> AMENKIEVNNKDEMNRWFEEFKKGNGLVDTFTNSYSFCESIPNLDRFVFQMASATDDAQKDSIYASALVEATKFCAPIYECAWVSSTGIVKKGLEWFEKNAGTIKSWDESYTELKVDVPKIEQLTGYQQAALKWRKDIGFRVNANTAALSNKVLAEYKVPGEIVMSVKEMLSDMIRRRNLILNRGGDENPRGPVSHEHVDWCREFVKGKYIMAFNPPWGDINKSGRSGIALVATGLAKLAETEGKGIFDEAKKTVEALNGYLDKHKDEVDRASADSMITNLLKHIAKAQELYKNSSALRAQSAQIDTAFSSYYWLYKAGVTPETFPTVSQFLFELGKQPRGTKKMKKALLSTPMKWGKKLYELFADDSFQQNRIYMHPAVLTAGRISEMGVCFGTIPVANPDDAAQGSGHTKSILNLRTNTETNNPCAKTIVKLFEVQKTGFNIQDMDIVASEHLLHQSLVGKQSPFQNAYNVKGNATS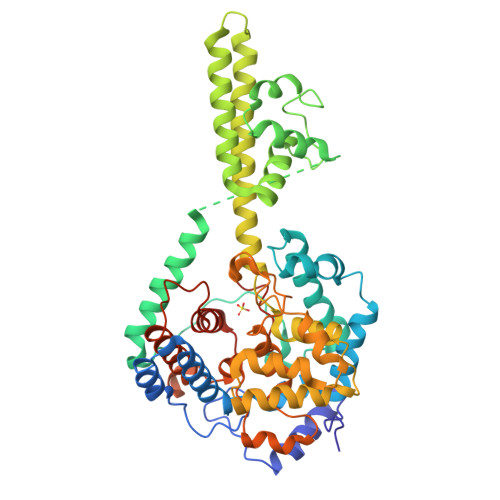ANII> MDGGMWLMQQINGQVARMKSLGMQLEAADIYNPNGSSLKDAVVMFDGGCTGVLVSNQGLLLTNHHCGYDQIQKHSSVQHNYLKDGFWSYSLAEELVNPGLEVEIVDEITDVTAAVKKELERIKKPSGLEFLSPRYLSSLAPEIVGKKAASRPGYRYEIKAFYGGNRYYMFTKKVFRDVRLVAAPPSSIGKFGSDTDNWAWPRHTGDFSIFRLYADKNGNPAEYSKDNVPYRPKRWVKVNAQGVKEGDFALIMGYPGTTYKFFTADEVTEWSEIDNNIRIEMRGILQDVMLREMLADPKINIMYAAKYASSQNGYKRAQGANWAIRRRSLREIKLAQQQEVLAWAKQKGIATTEEAVRAISKAIEGRQDLRMRQRYLLEGILMGIEMSNAPAADSDIADHWDDPARREAGLQSIRKQFEAFFNKDYSPEVEKDQLAIALLTRYAERIPAEKQPISIREGIAEYGSAKAYVEMIFDKSIYASRERFEEFMKNPDRDRLLRDPMSRFAASVAYEHQKLAKEVAAFDAPLAAAQRSYVASVLDMKGQPNLAPDANLTLRFTYGEIKGYQPRDVVTYGAKSTLEGVMEKEDPNNWEYVVDPKLKALYEAKNYGRYANSDGSMPVNFCATTHTTGGNAGSPVMNARGELIGLNFDRNWEGVGGDIEYLPNYQRSIILDIRYLLFIIDKFAGCQRLIDEIQPQFHHHHHH

Here, we show that dipeptidyl peptidase 11 (DPP11), a central metabolic enzyme in these bacteria, undergoes a conformational change upon peptide binding to distinguish substrates from end products. As previously reported, the overall fold of DPP11 comprises a bilobal architecture. The upper helical domain dictates the specificity of the enzyme and caps the catalytic domain, which has a typical chymotrypsin double β-barrel fold. The active site of DPP11 lays in a wide cleft running through the middle of the protein between the catalytic and helical domains, which contributes to the formation of the substrate binding subsites.

Interestingly, we obtained an unbound PeDPP11 crystal form, called here PeDPP11altconf, which lacks electron density for helix α14, indicating its susceptibility to unfold. Similar to PeDPP11 complexes, this structure is also closed (rotation angle of 27° of helical domain relative to the catalytic domain), illustrating the enzyme flexibility. The helical domain displays a high diversity of structural states across all solved structures in this work.>[4x]SPLAAYEVDDSTGYLTSDVGGPIQDQTSLKAGIRGPTLLEDFMFRQKIQHFDHERVPERAVHARGAGAHGTFTSYADWSNITAASFLNATGKQTPVFVRFSTVAGSRGSADTARDVHGFATRFYTDEGNFDIVGNNIPVFFIQDAIQFPDLIHSVKPRPDNEIPQAATAHDSAWDFFSQQPSTMHTLFWAMSGHGIPRSYRHMDGFGVHTFRFVKDDGSSKLIKWWFKSRQGKASLVWEEAQVLSGKNADFHRQDLWDAIESGNGPEWDVCVQIVDESQAQAFGFDLLDPTKIIPEEYAPLTKLGLLKLDRNPTNYFAETEQVMFQPGHIVRGIDFTEDPLLQGRLFSYLDTQ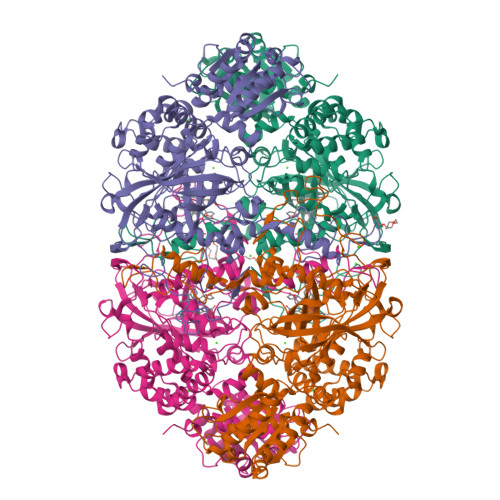LNRNGGPNFEQLPINMPRVPIHNNNRDGAGQMFIHRNKYPYTPNTLNSGYPRQANQNAGRGFFTAPGRTASGALVREVSPTFNDHWSQPRLFFNSLTPVEQQFLVNAMRFEISLVKSEEVKKNVLTQLNRVSHDVAVRVAAAIGLGAPDADDTYYHNNKTAGVSIVGSGPLPTIKTLRVGILATTSESSALDQAAQLRTRLEKDGLVVTVVAETLREGVDQTYSTADATGFDGVVVVDGAAALFASTASSPLFPTGRPLQIFVDAYRWGKPVGVCGGKSSEVLDAADVPEDGDGVYSEESVDMFVEEFEKGLATFRFTDRFALDS> MSSTMKDTQEAPVRWSRNWTPDAIRALVDQDNGKLDARIYADQDLYQLELERVFGRSWLMLGHETHIPKIGDYLTTYMGEDPVIMVRQKDQSIK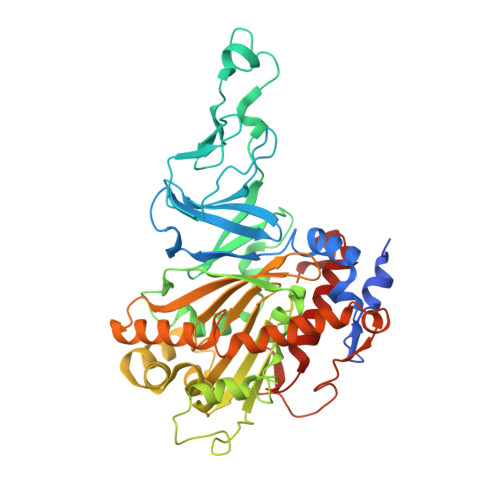VFLNQCRHRGMRIVRSDGGNAKAFTCTYHGWAYDIAGNLVNVPFEKEAFCDKKEGDCGFDKADWGPLQARVETYKGLVFANWDPEAPDLKTYLSDAMPYMDVMLDRTEAGTEAIGGIQKWVIPCNWKFAAEQFCSDMYHAGTMSHLSGVLAGLPPEMDLTQIQLSKNGNQFRSAWGGHGAGWFINDSSILLSVVGPKITQYWTQGPAAEKAARRVPQLPILDMFGQHMTVFPTCSFLPGINTIRTWHPRGPNEVEVWAFVLVDADAPEDIKEEFRLQNIRTFNAGGVFEQDDGENWVEIQRVMRGHKAKSTSLCAKMGLNVPNKNNPAYPGKTAYVYAEEAARGMYHHWSRMMSEPSWDTLKP>[2x]MPVDKNLRDLEPGIHTDLEGRLTYGGYLRLDQLLSAQQPLSEPAHHDEMLFIIQHQTSELWLKLLAHELRA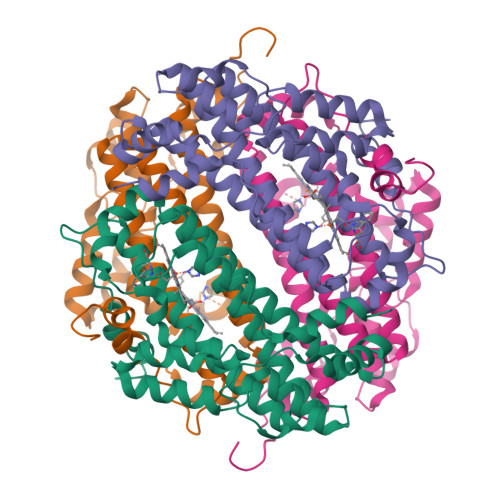AIVHLQRDEVWQCRKVLARSKQVLRQLTEQWSVLETLTPSEYMGFRDVLGPSSGFQSLQYRYIEFLLGNKNPQMLQVFAYDPAGQARLREVLEAPSLYEEFLRYLARFGHAIPQQYQARDWTAAHVADDTLRPVFERIYENTDRYWREYSLCEDLVDVETQFQLWRFRHMRTVMRVIGFKRGTGGSSGVGFLQQALALTFFPELFDVRTSVGVDNRPPQGSADAGKRLEHHHHHH> KPEFDPILLRPVDDLELTVRSANCLKAEAIHYIGDLVQ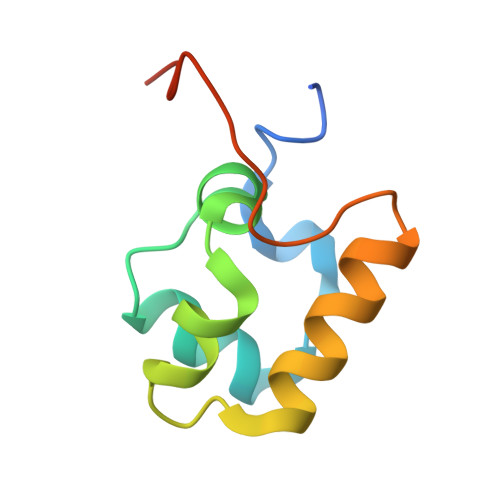RTEVELLKTPNLGKKSLTEIKDVLASRGLSLGMRLENWPPASIADE>[2x]GSHMTGELEVKNMDMKPGSTLKITGSIADGTDGFVINLGQGTDKLNLHFNPRFSESTIVCNSLDGSNWGQEQREDHLCFSPGSEVKFTVTFESDKFKVKLPDGHELTFPNRLGHSHLSYL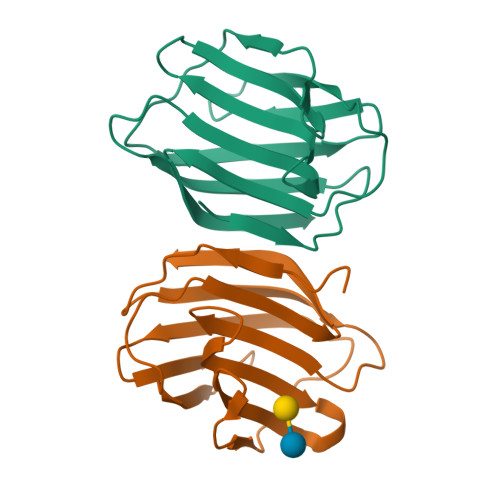SVRGGFNMSSFKLKE> NMEGDALHSLRANLVDPNNVLQSWDPTLVNPCTWFHVTCN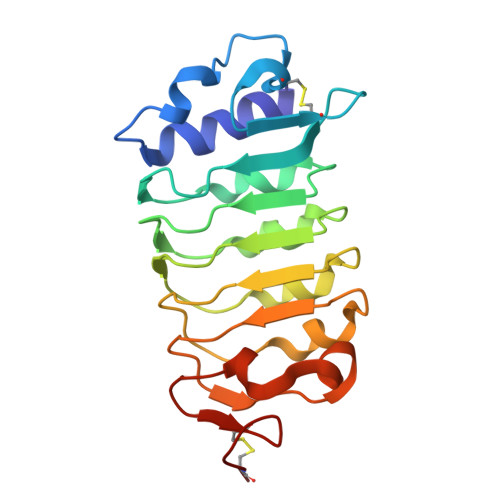NENSVIRVDLGNADLSGQLVPQLGQLKNLQYLELYSNNITGPVPSDLGNLTNLVSLDLYLNSFTGPIPDSLGKLFKLRFLRLNNNSLTGPIPMSLTNIMTLQVLDLSNNRLSGSVPDNGSFSLFTPISFANNLDLCGPVTSRPCP> MAELISKEGNKVEFKVSVPAAEVNRAYDQVWAGLARDVRVPGFRPGKAPRKVIENRVGKGYVESQVRDRLLETHYSQGLRELGLNLVDATVDPQDVQSGQAFEFTVKGETYP;> MSHYDILQAPVISEKAYSAMERGVYSFWVSPKATKTEIKDAIQQAFGVRVIGISTMNVPGKRKRVGRFIGQRNDRKKAIVRLAEGQSIEALAGQA;> MPRPSAGSHHNDKLHFKKGDTVIVLSGKHKGQTGKVLLALPRDQKVVVEGVNVITKNVKPSMTNPQGGQEQRELALHASKVALVDPETGKATRVRKQIVDGKKVRVAVASGKTID;> MKPSEMRNLQATD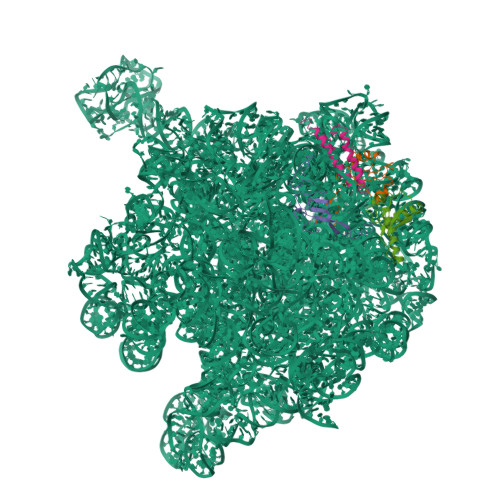FAKEIDARKKELMELRFQAAAGQLAQPHRVRQLRREVAQLNTVKAELARKGEQQ4,6-O-[(1S)-1-carboxyethylidene]-beta-D-glucopyranose | C9 H14 O8 | 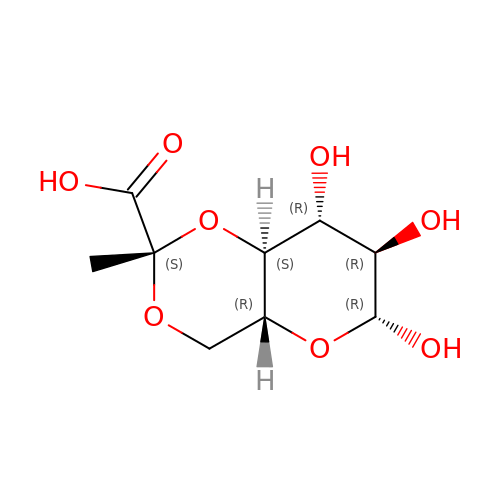QVVFNJUJKXWFAU-GLPGPYIRSA-N> MHHHHHHSSGRENLYFQGDTMQPIERKRQGYIHELIQTEERYMADLQLVVEVFQKRMAE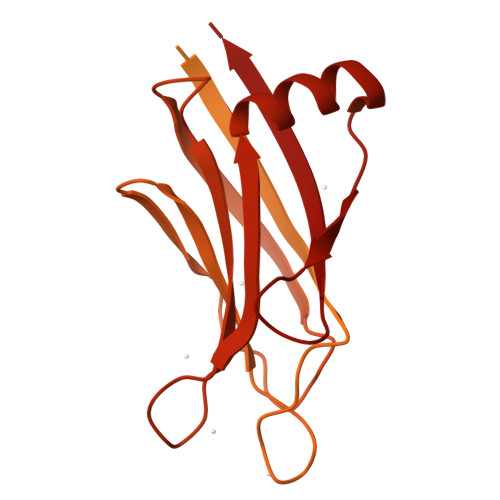SGFLTEGEMALIFVNWKELIMSNTKLLKALRVRKKTGGEKMPVQMIGDILAAELSHMQAYIRFCSCQLNGAALLQQKTDEDTDFKEFLKKLASDPRCKGMPLSSFLLKPMQRITRYPLLIRSILENTPESHADHSSLKLALERAEELCSQVNEGVREKENSDRLEWIQAHVQCEGLAEQLIFNSLTNCLGPRKLLHSGKLYKTKSNKELHGFLFNDFLLLTYMVKQFAVSSGSEKLFSSKSNAQFKMYKTPIFLNEVLVKLPTDPSSDEPVFHISHIDRVYTLRTDNINERTAWVQKIKAASEQYIDTEKKQREKAYQARSQKTSGIGRLMVHVIEATELKACKPNGKSNPYCEISMGSQSYTTRTIQDTLNPKWNFNCQFFIKDLYQDVLCLTLFDRDQFSPDDFLGRTEIPVAKIRTEQESKGPMTRRLLLHEVPTGEVWVRFDLQLFE>[2x]MHHHHHHSTATNPLDLDVCAREPIHIPGLIQPYGVLLVIDPADGRIVQASTTAADLLGVPMAALLGMPYTQVLTLPEAQPFAVDDQPQHLMHAEVRFPQRATPPASAWVAAWHLYPQQWLVEMEPRDARLLDVTLREAMPLLRSVERDPGIAEAAVRVAKGLRSLIGFDRVMIYRFDEEWNGDIIAEARKPELEAYLGLHYPASAIPAQARALYLRNRVRQIADVGYQPSPIQPTVHPQLGTPVDLSDVSLRSVSPVHLEYLANMGVTATLVASIVVNDALWGLISCHHYSPHFTNHAMRDVTDAVARTLAGRIGALQAVARARLESVLLTVREKLITDFNDAEHMTVELLDDMAPDLMDVVDADGVAIFHGNDISRHGTTPDVAALRR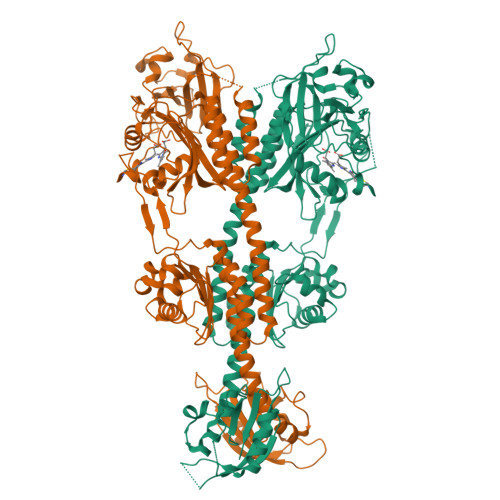IRDHIESEHHEALREDAVGALHVDAIGEVFPELADLAPLAAGFIFVPLMPQSRSALLWTRREQIQQIKWAGNPQLAKLEDIPNSRLSPRKSFDLWQQTVRGRARRWSPLHLESARSLRVLIELMERKRFQQDFTLLEASLSRLRDGVAIIERGTANAAHRLLFVNTAFADVCGSDVAELIGRELQTLYASDAPRANVELLQDALRNGRAAYVTLPLQVSDGAPVYRQFHLEPLPSPSGVTAHWLLQLRDPE>[2x]MNNTIETILAHRSIRKFTAVPITDEQRQTIIQAGLAASSSSMLQVVSIVRVTDSEKRNELAQFAGNQAYVESAAEFLVFCIDYQRHATINPDVQADFTELTLIG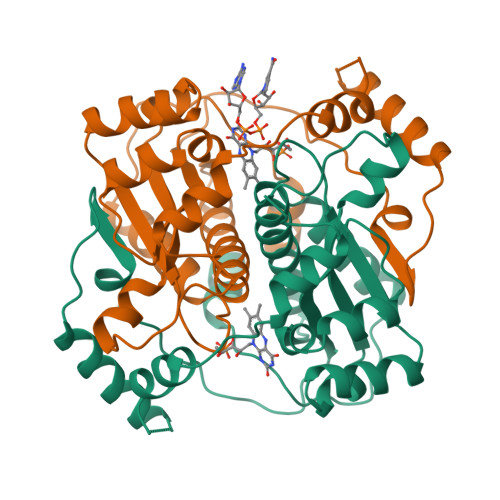AVDSGIMAQNCLLAAESMGLGGVYIGGLRNSAAQVDELLGLPENSAVLFGMCLGHPDQNPEVKPRLPAHVVVHENQYQELNLDDIQSYDQTMQAYYASRTSNQKLSTWSQEVTGKLAGESRPHILPYLNSKGLAKR>MSLTVQKINWEQVKEWDRKYLMRTFSTQNEYQPVPIESTEGDYLIMPDGTRLLDFFNQLYCVNLGQKNQKVNAAIKEALDRYGFVWDTYATDYKAKAAKIIIEDILGDEDWPGKVRFVSTGSEAVETALNIARLYTNRPLVVTREHDYHGWTGGAATVTRLRSYRSGLVGENSESFSAQIPGSSYNSAVLMAPSPNMFQDSDGNLLKDENGELLSVKYTRRMIENYGPEQVAAVITEVSQGAGSAMPPYEYIPQIRKMTKELGVLWINDEVLTGFGRTGKWFGYQHYGVQPDIITMGKGLSSSSLPAGAVLVSKEIAAFMDKHRWESVSTYAGHPVAMAAVCANLEVMMEENFVEQAKDSGEYIRSKLELLQEKHKSIG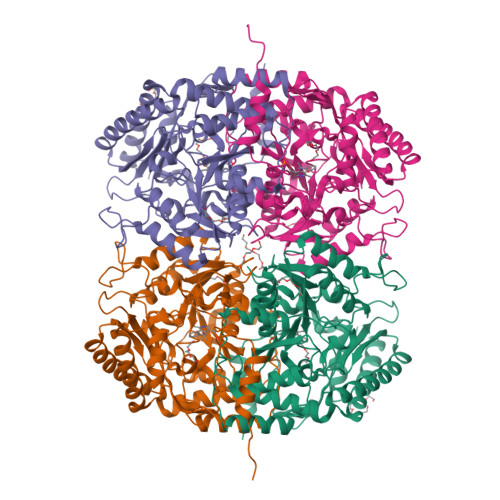NFDGYGLLWIVDIVNAKTKTPYVKLDRNFTHGMNPNQIPTQIIMKKALEKGVLIGGVMPNTMRIGASLNVSRGDIDKAMDALDYALDYLESGEWQALEHHHHHH[4x]>MEKFLVIAGPCAIESEELLLKVGEEIKRLSEKFKEVEFVFKSSFDKANRSSIHSFRGHGLEYGVKALRKV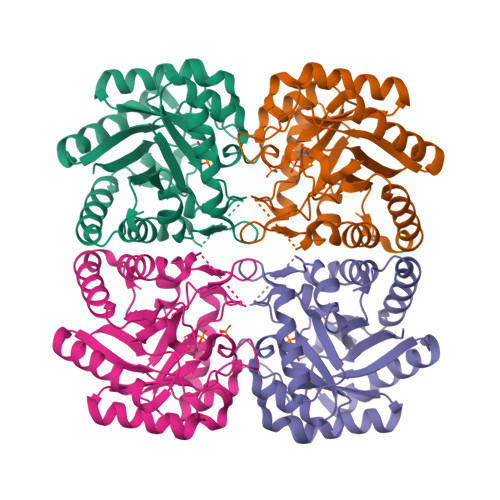KEEFGLKITTDIHESWQAEPVAEVADIIQIPAFLCGQTDLLLAAAKTGRAVNVKKGQFLAPWDTKNVVEKLKFGGAKEIYLTERGTTFGYNNLVVDFRSLPIMKQWAKVIYDATHSVQLPGGLGDKSGGMREFIFPLIRAAVAVGCDGVFMETHPEPEKALSDASTQLPLSQLEGIIEAILEIREVASKYYETIPVK[2x]>[2x]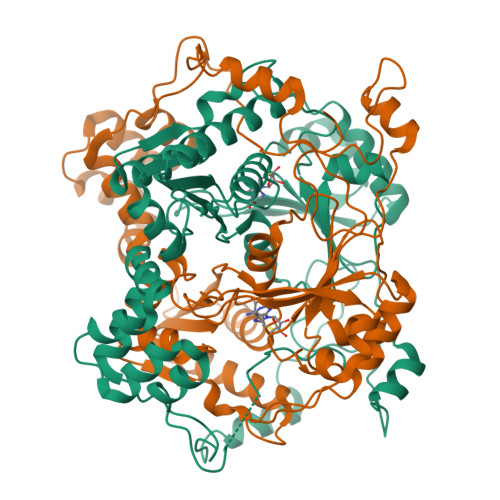GTSTQTKAGSLTIVGTGIESIGQMTLQALSYIEAAAKVFYCVIDPATEAFILTKNKNCVDLYQYYDNGKSRLNTFTQMSELMVREVRKGLDVVGVFYGHPGVFVNPSHRALAIAKSEGYRARMLPGVSAEDCLFADLCIDPSNPGCLTYEASDFLIRDRPVSIHSHLVLFQVGCVGIADFNFTGFDNNKFGVLVDRLEQEYGAEHPVVHYIAAMMPHQDPVTDKYTVAQLREPEIAKRVGGVSTFYIPPKARKASNLDIIRRLELLPAGQVPDKKARIYPANQWEPDVPEVEPYRPSDQAAIAQLADHAPPEQYQPLATSKAMSDVMTKLALDPKALADYKADHRAFAQSVPDLTPQERAALELGDSWAIRCAMKNMPSSLLDAARESGEEASQNGFPWVIVVGVIGVIG>[3x]GAPAAVDWRARGAVTAVKDQGQCGSCWAFSAIGNVECQWFLAGHPLT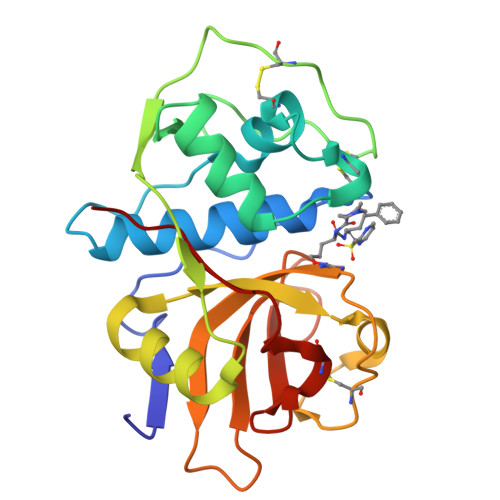NLSEQMLVSCDKTDSGCSGGLMNNAFEWIVQENNGAVYTEDSYPYASGEGISPPCTTSGHTVGATITGHVELPQDEAQIAAWLAVNGPVAVAVDASSWMTYTGGVMTSCVSEQLDHGVLLVGYNDSAAVPYWIIKNSWTTQWGEEGYIRIAKGSNQCLVKEEASSAVVG> SNAMAALPDKEKLLRNFTRCANWEEKYLYIIELGQRLAELNPQDR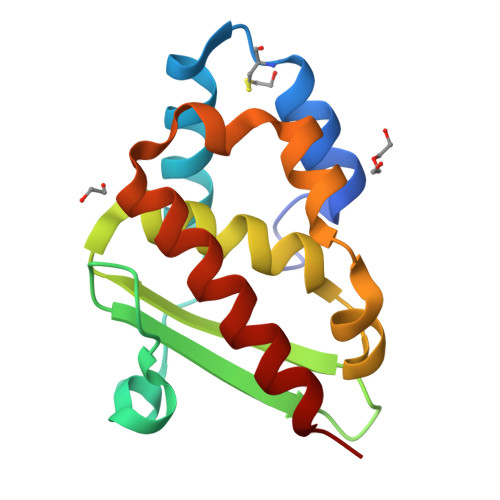NPQNTIHGCQSQVWIVMRRNANGIIELQGDSDAAIVKGLMAVVFILYHQMTAQDIVHFDVRPWFEKMALAQHLTPSRSQGLEAMIRAIRAKAATLS>[2x]MFSAGHKIKGTVVLMPKNELEVNPDGSAVDNLNAFLGRSVSLQLISATKADAHGKGKVGKDTFLEGINTSLPTLGAGESAFNIHFEWDGSMGIPGAFYIKNYMQVEFFLKSLTLEAISNQGTIRFVCNSWVYNTKLYKSVRIFFANHTYVPSETPAPLVEYREEELKSLRGNGTGERKEYDRIYDYDVYNDLGNPDKSEKLARPVLGGSSTFPYPRRGRTGRGPTVTDPNTEKQGEVFYVPRDENLGHLKSKDALEIGTKSLSQIVQPAFESAFDLKSTPIEFHSFQDVHDLYEGGIKLPRDVISTIIPLPVIKELYRTDGQHILKFPQPHVVQVSQSAWMTDEEFAREMIAGVNPCVIRGLEEFPPKSNLDPAIYGDQSSKITADSLDLDGYTMDEALGSRRLFMLDYHDIFMPYVRQINQLNSAKTYATRTILFLREDGTLKPVAIELSLPHSAGDLSAAVSQVVLPAKEGVESTIWLLAKAYVIVNDSCYHQLMSH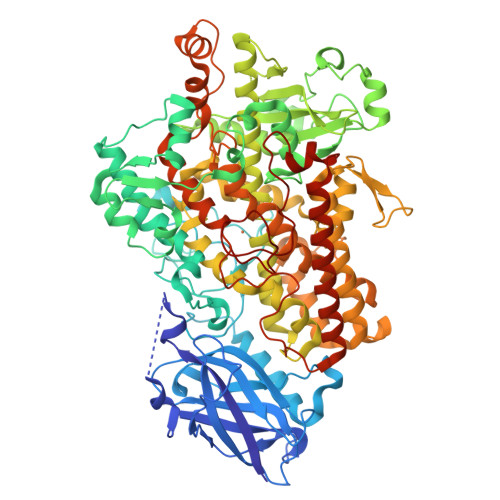WLNTHAAMEPFVIATHRHLSVLHPIYKLLTPHYRNNMNINALARQSLINANGIIETTFLPSKYSVEMSSAVYKNWVFTDQALPADLIKRGVAIKDPSTPHGVRLLIEDYPYAADGLEIWAAIKTWVQEYVPLYYARDDDVKNDSELQHWWKEAVEKGHGDLKDKPWWPKLQTLEDLVEVCLIIIWIASALHAAVNFGQYPYGGLIMNRPTASRRLLPEKGTPEYEEMINNHEKAYLRTITSKLPTLISLSAIEILSTHASDEVYLGQRDNPHWTSDSKALQAFQKFGNKLKEIEEKLVRRNNDPSLQGNRLGPVQLPYTLLYPSSEEGLTFRGIPNSISI> MVTENPQRLTVLRLATNKGPLAQIWLASNMSNIPRGSVIQTH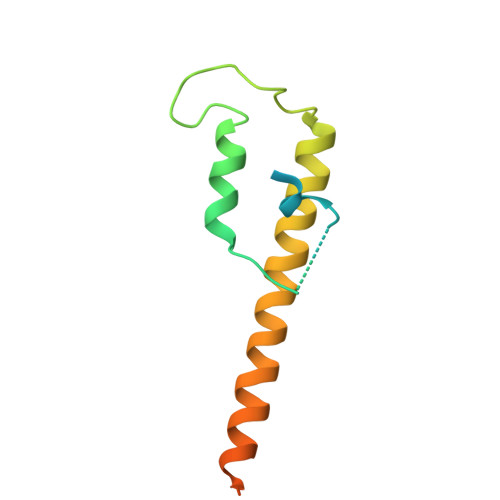IAESAKEIAKASGCDDESGDNEYITLRTSGELLQGIVRVYSKQATFLLTDIKDTLTKISMLFKTSQKMTSTVNHHHHHH> 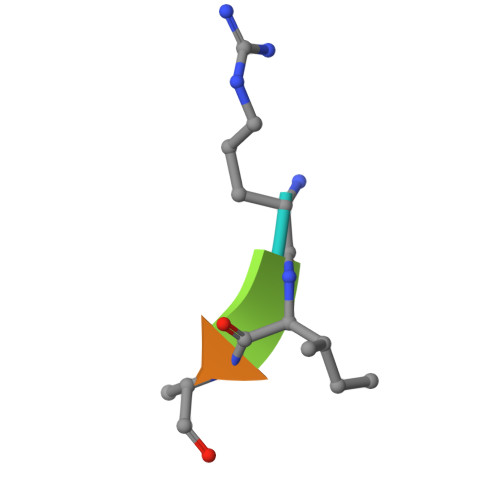RIAAA>[4x]SMMELRVGNRYRLGRKIGSGSFGDIYLGTDIAAGEEVAIKLECVKTKHPQLHIESKIYKMMQGGVGIPTIRWCGAEGDYNVMVMELLGPSLEDLFNFCSRKFSLKTVLLLADQMISRIEYIHSKNFIHRDVKPDNFLMGLGKKGNLVYIIDFGLAKKYRDARTHQH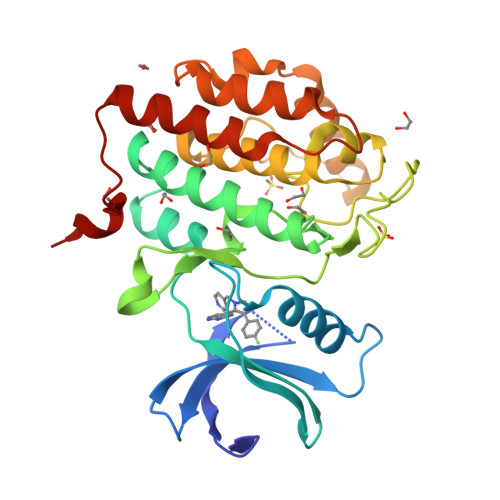IPYRENKNLTGTARYASINTHLGIEQSRRDDLESLGYVLMYFNLGSLPWQGLKAATKRQKYERISEKKMSTPIEVLCKGYPSEFATYLNFCRSLRFDDKPDYSYLRQLFRNLFHRQGFSYDYVFDWNMLK>MVPELKQISRVEAMRLGPGWSHSCHAMLYAANPGQLFGRIPMRFSVLMQMRFDGLLGFPGGFVDRRFWSLEDGLNRVLGLGLGCLRLTEADYLSSHLTEGPHRVVAHLYARQLTLEQLHAVEISAVHSRDHGLEVLGLVRVPLYTQKDRVGGFPNFLSNAFVSTAKCQLLFALKVLNMMPEEKLVEALAAATEKQKKALEKLL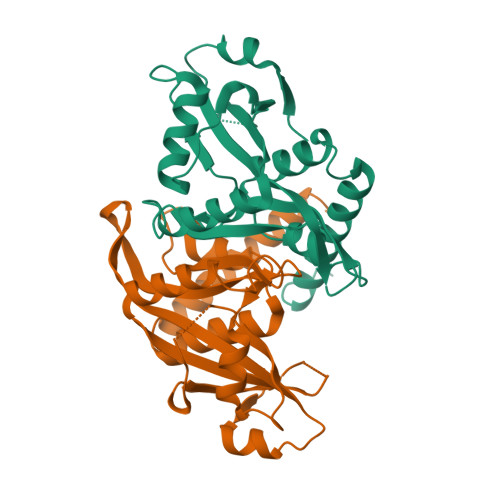PASS[2x]> MDLTLIIDNYDSFVYNIAQIVGELGSYPIVIRNDEISIKGIERIDPDRLIISPGPGTPEKREDIGVSLDVIKYLGKRTPIL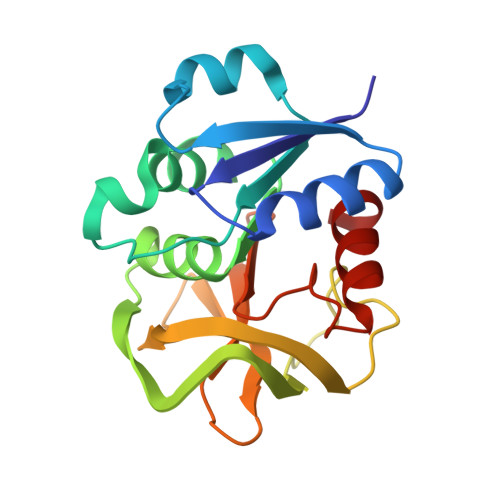GVCLGHQAIGYAFGAKIRRARKVFHGKISNIILVNNSPLSLYYGIAKEFKATRYHSLVVDEVHRPLIVDAISAEDNEIMAIHHEEYPIYGVQFHPESVGTSLGYKILYNFLNRV>MSIADIAFIDAAFTRTPEARANYLAVTRAALEGRLALFAARLARHSEAEVAATIDPGFLLDILDLLYSLPAALREALPAEVQARIALFEAFLARYADHPNLALVGRVFREIQAIRAKYSGKLPDEYINTLALIRVDRARLVRDMRLVEETAVIVAAYALAFDPPERHPEAEARMRATIERANALRRAAGFPPSLAPE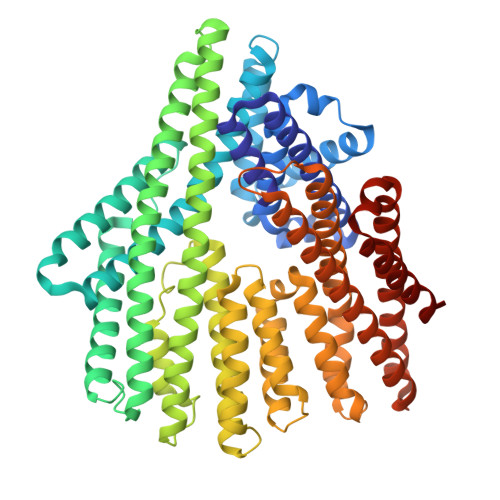EGLARARRLAARLRALRAAVRARRLPTGVPLTPEQAAAILATLERLYEVALEIGRAIDAYLAAAEAYAATAAELEANGASLDPAARAALMEATLRARGAVIRERAALLRLLRRFYALVLELDFLLLRAYAEAGHDPDDPALLALLRELDPFNGMTTSELHRRRRRLRDLYIDLVAAMLRGVKNGELTWEEVVAIMDGLLARLADPEVSEEEALVGLLEEIVKDKKPIAEKALKIAVDFVEANPEFLRDGRAGLALIRVVLEYALDDPDAHKELVAFAAAHLPRALDAAVDEIRDLLNDVRILFHSKPSPFLSAEEQKALAKKKLKQVKEILDLMKEIAELAKKIKAKSKDPEVKALMDAMLADIQAAAKEIAKHLEELLKDKELAAAFPELKTLLKLAKEIVKMLEHHHHHH[3x]>[2x]MYTMGLDIGSTASKGVILKNGEDIVASETISSGTGTTGPSRVLEKLYGKTGLAREDIKKVVVTGYGRMNYSDADKQISELSCHARGVNFIIPETRTIIDIGGQDAKVLKLDNNGRLLNFLMNDKCAAGTGRFLDVMAKIIEVDVSELGSISMNSQNEVSISSTCTVFA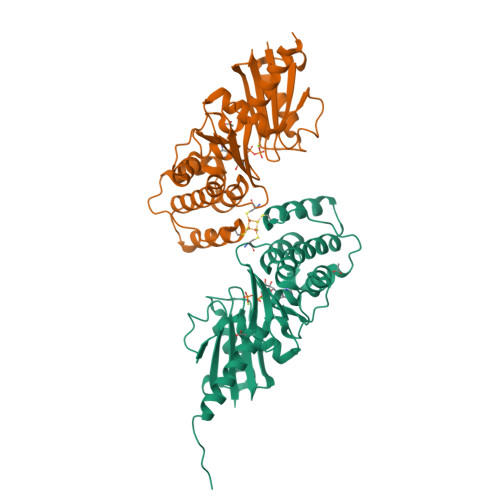ESEVISHLSENAKIEDIVAGIHTSVAKRVSSLVKRIGVQRNVVMVGGVARNSGIVRAMAREINTEIIVPDIPQLTGALGAALYAFDEAKESQKEVKNISAWSHPQFEK>[8x]MIRNGFYIIKDRFFSDMSDPYLKGNKKQNRPHYYCFEDSNYNGIYWMIPLSSRIDKYKKIVSKRTGKGRNCDIIHIVKLDDSHESAFLIQDMFPISDKYIEREYTIAGNHLRLTSEHAAKEIEQKARKVLGMLKRGIKFTPTQPDIQKIYERLQQ

The focus of the present study, Type III systems, comprise a ribonuclease (RNase) toxin that processes, and is then directly inhibited by, its structured and specific cognate RNA antitoxin. Over 120 putative Type III TA loci have been identified bioinformatically, in very diverse bacterial species, and these systems fall into three separate families (named ToxIN, CptIN and TenpIN) based on sequence similarity of their toxin components. Many Type III TA systems are plasmid-encoded but we decided to investigate the chromosomally-encoded CptIN system, from the human commensal Eubacterium rectale (CptINEr) as the first representative of the CptIN family. The RNA chains seen in the CptIN complex structure each correspond to single repeats from the repetitive CptI sequence and a cyclic phosphate is seen at the 3′ end of each RNA chain on the A45 nucleotide; these observations indicate that the CptN protein is, like ToxN, a ribonuclease that processes its own antitoxin.

The best diffracting crystals (1 native and 2 SeMet) were isomorphous, and, following phasing through SAD, the final structure was solved to a resolution of 2.2 Å. The unit cell contained a total of eight protein (CptNEr) monomers each complexed with a single CptIEr RNA repeat of 45 nt. Examination of the symmetry units reveals that each protein–RNA heterodimer formed a self-closing, heterotetrameric ring-shaped complex with a heterodimer from the neighbouring asymmetric unit. The heterotetrameric architecture is a major deviation from the heterohexameric complexes formed by the other structurally-defined Type III TA systems. The structural core of the CptN protein is similar to the structures of the three previously solved Type III toxins, being made up of a highly twisted antiparallel β-sheet. Of note is the absence of the kink in the third helix that is seen in the structures of ToxNPa, ToxNBt and AbiQ; the equivalent helix H4 in CptNEr is visibly shorter in comparison and, as a result, CptNEr more closely resembles the structure of the Type II Toxin Kid. Each CptNEr protein binds two CptIEr RNAs, and the protein–RNA interfaces are considerable for both. The CptIEr RNA observed bound to CptNEr is a classic H-type pseudoknot of 45 nt, which is derived from the two genetic cptIEr repeats. While the Pectobacterium and Bacillus ToxI structures are very similar to each other, the fold of the CptIEr differs markedly from the ToxI paradigm, and is also structurally extremely unusual among known RNA pseudoknots notably in the structure of the loops. L2 forms a short, three-stranded helix which has been previously referred to as an A-minor twist motif.> MNYNNKILVSESGLSQKHLIHGDEELFQHELKTIFARNWLFLTHDSLIPAPGDYVTAKMGIDEVIVSRQNDGSIRAFLNVCRHRGKTLVSVEAGNAKGFVCSYHGWGFGSNGELQSVPFEKDLYGESLNKKCLGLKEVARVESFHGFIYGCFDQEAPPLMDYLGDAAWYLEPMFKHSGGLELVGPPGKVVIKANWKAPAENFVGDAYHVGWTHASSLRSGESIFSSLAGNAALPPEGAGLQMTSKYGSGMGVLWDGYSGVHSADLVPELMAFGGAKQERLNKEIGDVRARIYRSHLNCTVFPNNSMLTCSGVFKVWNPIDA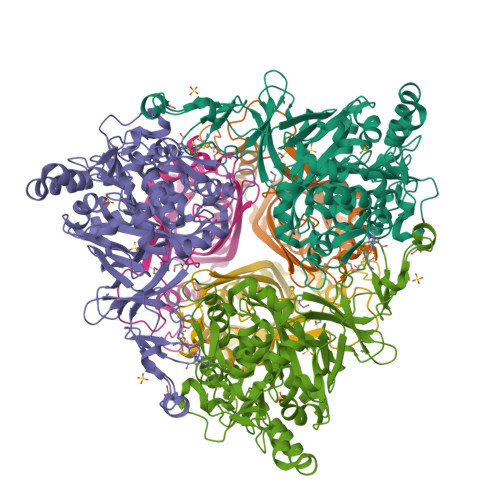NTTEVWTYAIVEKDMPEDLKRRLADSVQRTFGPAGFWESDDNDNMETASQNGKKYQSRDSDLLSNLGFGEDVYGDAVYPGVVGKSAIGETSYRGFYRAYQAHVSSSNWAEFEHASSTWHTELTKT;> INIQEDKLVSAHDAEEILRFFNCHDSALQQEATTLLTQEAHLLDIQAYRAWLEHCVGSEVQYQVISRELRAASERRYKLNEAMNVYNENFQQLKVRVEHQLDPQNWGNSPKLRFTRFITNVQAAMDVNDKELLHIRSNVILHRARRGNQVDVFYAAREDKWKRGEGGVRKLVQRFVDYPERILQTHNLMVFL>SNAMSEWSRIAVEFGEQQLNLTELEDFARELAYEGLDPALIIKKLKETGGDDWVKDTKFIIVFALTRGNKIVKASGKMSNSGSKRLMALQEKYGLVERAETRLSITPVRVAQSLPTWTCAAAAALKEYLPVG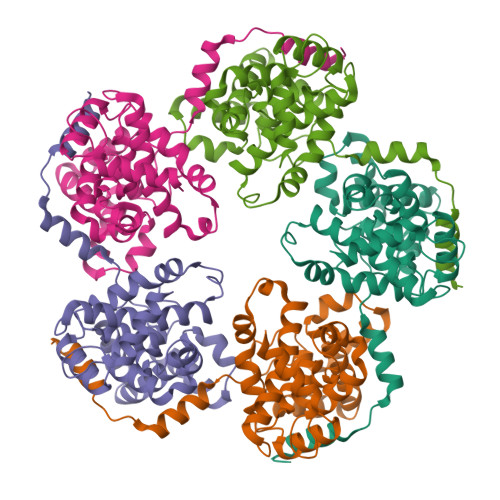PAVMNLKVENYPPEMMCMAFGSLIPTAGVSEATTKTLMEAYSLWQDAFTKTINVKMRGASKTEVYNSFRDPLHAAVNSVFFPNDVRVKWLKAKGILGPDGVPSRAAEVAAAAYRNL[5x]propyl 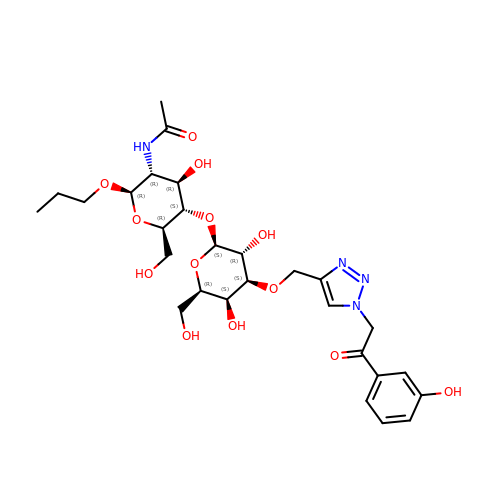2-(acetylamino)-2-deoxy-4-O-[3-O-({1-[2-(3-hydroxyphenyl)-2-oxoethyl]-1H-1,2,3-triazol-4-yl}methyl)-beta-D-galactopyranosyl]-beta-D-glucopyranoside | C28 H40 N4 O13 | ABYAFHNJWAOAFG-ONVHQJCOSA-N> MASMTGGQQMGRDQAGITGTWYNQLGSTFIVTAGADGALTGTYESAVGNAES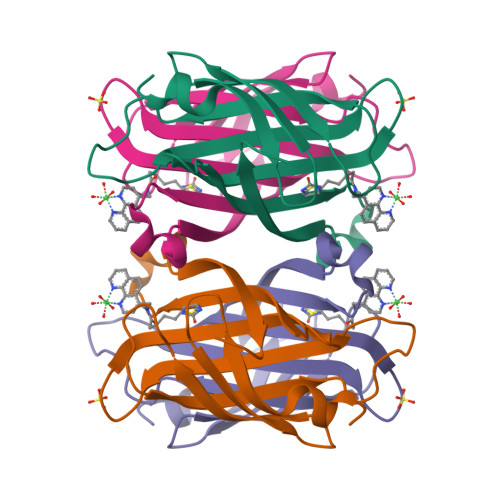RYVLTGRYDSAPATDGSGTALGWTVAWKNNYRNAHSATTWSGQYVGGAEARINTQWLLTVGTTEANAWKSTLVGHDTFTKVKPSAASIDAAKKAGVNNGNPLDAVQQ>[2x]MTMMDMNFKYCHKIMKKHSKSFSYAFDLLPEDQRKAVWAIYAVCRKIDDSIDVYGDIQFLNQIKEDIQSIEKYPYEYHHFQSDRRIMMALQHVAQHKNIAFQSFYNLIDTVYKDQHFTMFETDAELFGYCYGVAGTVGEVLTPILSDHETHQTYDVARRLGESLQLINILRDVGEDFENERIYFSKQRLKQYEVDIAEVYQNG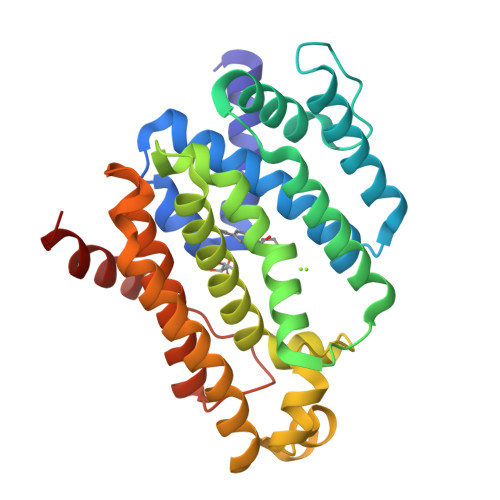VNNHYIDLWEYYAAIAEKDFRDVMDQIKVFSIEAQPIIELAARIYIEILDEVRQANYTLHERVFVEKRKKAKLFHEINSKYHRI> PKCIQCGQYLDDPDLKYGQHPPDAVDEPQMLTNEKLSIFDANESGFESYEALPQHKLTCFSVYCKHGHLCPIDTGLIEKNIELFFSGSAKPIYDDDPSLEGGVNGKNLGPINEWWITGFDGGEKALIGFSTSFAEYILMDPSPEYAPIFGLMQEKIYISKIVVEFLQSNSDSTYEDLINKIETTVPPSGLNL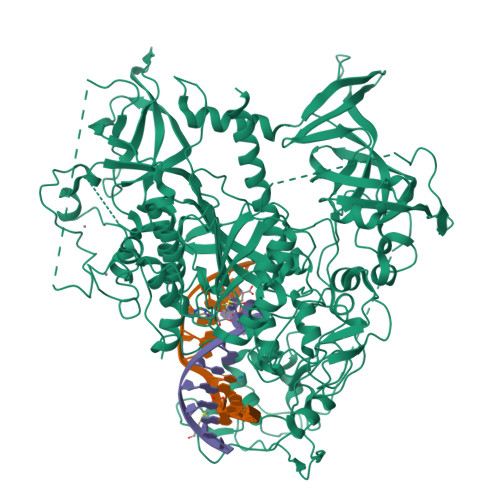NRFTEDSLLRHAQFVVEQVESYDEAGDSDEQPIFLTPCMRDLIKLAGVTLGQRRAQARRQTIRHSTREKDRGPTKATTTKLVYQIFDTFFAEQIEKDDREDKENAFKRRRCGVCEVCQQPECGKCKACKDMVKFGGSGRSKQACQERRCPNMAMKEADDDEEVDDNIPEMPSPKKMHQGKKKKQNKNRISWVGEAVKTDGKKSYYKKVCIDAETLEVGDCVSVIPDDSSKPLYLARVTALWEDSSNGQMFHAHWFCAGTDTVLGATSDPLELFLVDECEDMQLSYIHSKVKVIYKAPSENWAMEGGMDPESLLEGDDGKTYFYQLWYDQDYARFESPPKTQPTEDNKFKFCVSCARLAEMRQKEIPRVLEQLEDLDSRVLYYSATKNGILYRVGDGVYLPPEAFTFNIKLSSPVKRPRKEPVDEDLYPEHYRKYSDYIKGSNLDAPEPYRIGRIKEIFCPKKSNGRPNETDIKIRVNKFYRPENTHKSTPASYHADINLLYWSDEEAVVDFKAVQGRCTVEYGEDLPECVQVYSMGGPNRFYFLEAYNAKSKSFEDPPNHARSPGNKGKGKGKGKGKPKSQACEPSEPEIEIKLPKLRTLDVFSGCGGLSEGFHQAGISDTLWAIEMWDPAAQAFRLNNPGSTVFTEDCNILLKLVMAGETTNSRGQRLPQKGDVEMLCGGPPCQGFSGMNRFNSRTYSKFKNSLVVSFLSYCDYYRPRFFLLENVRNFVSFKRSMVLKLTLRCLVRMGYQCTFGVLQAGQYGVAQTRRRAIILAAAPGEKLPLFPEPLHVFAPRACQLSVVVDDKKFVSNITRLSSGPFRTITVRDTMSDLPEVRNGASALEISYNGEPQSWFQRQLRGAQYQPILRDHICKDMSALVAARMRHIPLAPGSDWRDLPNIEVRLSDGTMARKLRYTHHDRKNGRSSSGALRGVCSCVEAGKACDPAARQFNTLIPWCLPHTGNRHNHWAGLYGRLEWDGFFSTTVTNPEPMGKQGRVLHPEQHRVVSVRECARSQGFPDTYRLFGNILDKHRQVGNAVPPPLAKAIGLEIKLCMLAKARESASAKIKEEEAAKD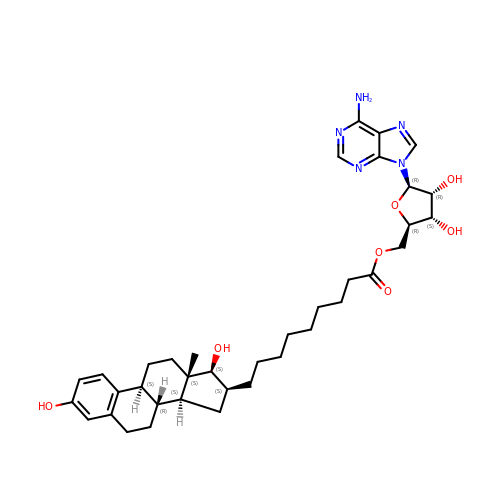O5'-[9-(3,17B-DIHYDROXY-1,3,5(10)-ESTRATRIEN-16B-YL)-NONANOYL]ADENOSINE | C37 H51 N5 O7 | CKSDYJASHNGOOS-KTXOUVACSA-N> SRGASNSSNNNNNNNKVYKRYNSKAKEISRHCVFCENNNEPEAVINSHSVRDNFNRVLCPKLRTYVCPICGASGDSAHTI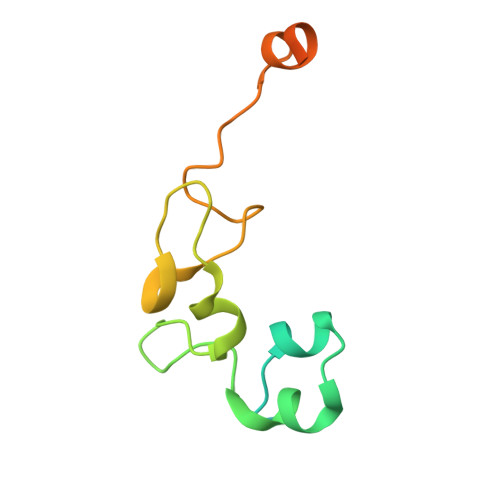KYCPKKPIITMEDAIKAESFRLAKSSYYKQQMKVV N-(2-AMINOETHYL)-5-CHLOROISOQUINOLINE-8-SULFONAMIDE | C11 H12 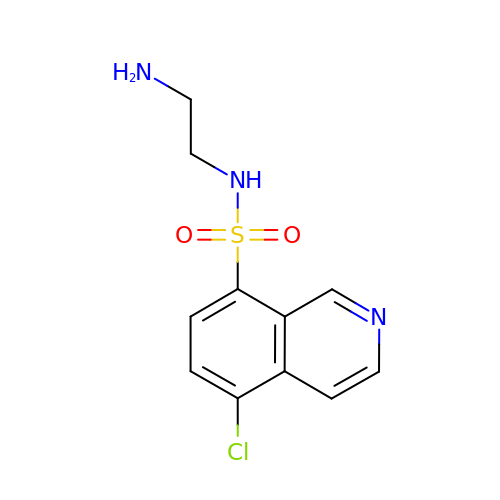Cl N3 O2 S | OGKYMFFYOWUTKV-UHFFFAOYSA-N> APDTSVSNKQNFSTDVIYQIFTDRFSDGNPANNPTGAAFDGTCTNLRLYCGGDWQGIINKINDGYLTGMGVTAIWISQPVENIYSIINYSGVNNTAYHGYWARDFKKTNPAYGTIADFQNLIAAAHAKNIKVIIDFAPNHTSPASSDQPSFAENGRLYDNGTLLGGYTNDTQNLFHHNGGTDFSTTENGIYKNLGDLADLNHNNSTVDVYLKDAIKMWLDLGIDGIRMDAVKHMPFGWQKSFMAAVNNYKPVFTFGEWFLGVNEVSPENHKFANESGMSLLDFRFAQKVRQVFRDNTDNMYGLKAMLEGSAADYAQVDDQVTF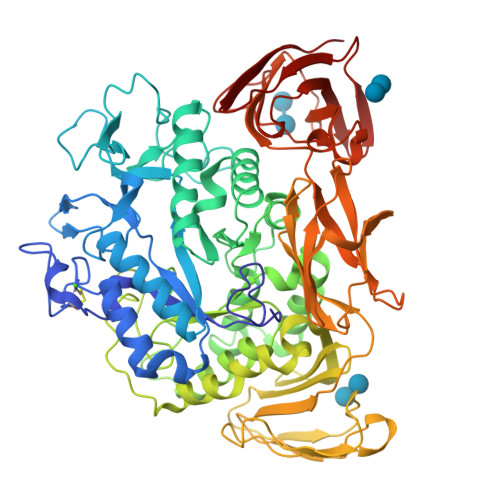IDNHDMERFHASNANRRKLEQALAFTLTSRGVPAIYYGTEQYMSGGTDPDNRARIPSFSTSTTAYQVIQKLAPLRKCNPAIAYGSTQERWINNDVLIYERKFGSNVAVVAVNRNLNAPASISGLVTSLPQGSYNDVLGGLLNGNTLSVGSGGAASNFTLAAGGTAVWQYTAATATPTIGHVGPMMAKPGVTITIDGRGFGSSKGTVYFGTTAVSGADITSWEDTQIKVKIPAVAGGNYNIKVANAAGTASNVYDNFEVLSGDQVSVRFVVNNATTALGQNVYLTGSVSELGNWDPAKAIGPMYNQVVYQYPNWYYDVSVPAGKTIEFKFLKKQGSTVTWEGGSNHTFTAPSSGTATINVNWQP>MSNGILSQSIANMQQAEATIQSFSGLPQNAVNIQQNVGEVVAALLPQVQTMQQQVLAFAARLELQLTQQLANTGPFNPEALKAFVDLVQQEIAPIQTLTAQTLTASQSANDRITQDNIALQRIGVELQATIAGLQSNLDGARQELDSLNKKKLYLLGLGLLGLPGLIALAVTLTQTQNKVSSLEGQVNQIEGQIQRQQGFLGQTTAFSQQFGSLIDRVSKVGNTISL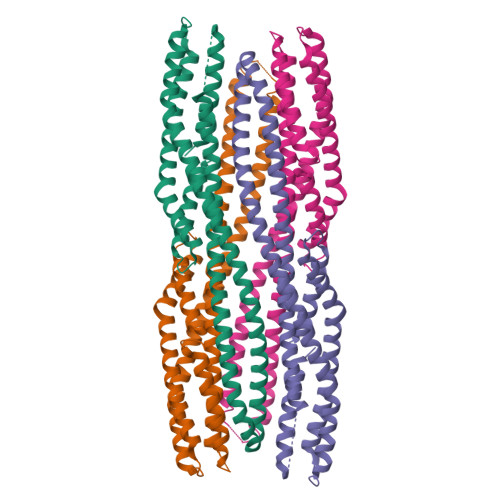LGGDIANVARDAGQGDPELARLFFTAALTEVRTLQVDASLEHHHHHH[2x]> MNPNNRSEHDTIKTTENNEVPTNHVQYPLAETPNPTLEDLNYKEFLRMTADNNTEALDSSTTKDVIQKGISV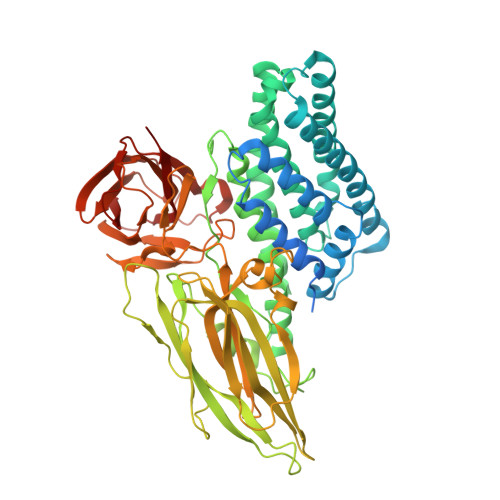VGDLLGVVGFPFGGALVSFYTNFLNTIWPSEDPWKAFMEQVEALMDQKIADYAKNKALAELQGLQNNVEDYVSALSSWQKNPVSSRNPHSQGRIRELFSQAESHFRNSMPSFAISGYEVLFLTTYAQAANTHLFLLKDAQIYGEEWGYEKEDIAEFYKRQLKLTQEYTDHCVKWYNVGLDKLRGSSYESWVNFNRYRREMTLTVLDLIALFPLYDVRLYPKEVKTELTRDVLTDPIVGVNNLRGYGTTFSNIENYIRKPHLFDYLHRIQFHTRFQPGYYGNDSFNYWSGNYVSTRPSIGSNDIITSPFYGNKSSEPVQNLEFNGEKVYRAVANTNLAVWPSAVYSGVTKVEFSQYNDQTDEASTQTYDSKRNVGAVSWDSIDQLPPETTDEPLEKGYSHQLNYVMCFLMQGSRGTIPVLTWTHKSVDFFNMIDSKKITQLPLVKAYKLQSGASVVAGPRFTGGDIIQCTENGSAATIYVTPDVSYSQKYRARIHYASTSQITFTLSLDGAPFNQYYFDKTINKGDTLTYNSFNLASFSTPFELSGNNLQIGVTGLSAGDKVYIDKIEFIPVN> FKAERLRVNLRLVINRLKLLEKKKTELAQKARKEIADYLAAGKDERARIRVEHIIREDYLVEAMEILELYCDLLLARFGLIQSMKELDSGLAESVSTLIWAAPRLQSEVAELKIVADQLCAKYSKEYGKLCRTNQIGTVNDRL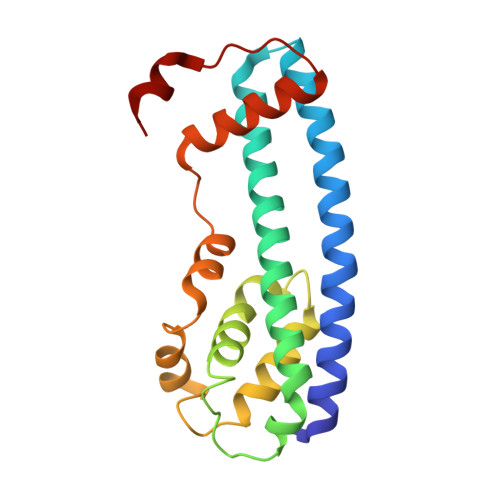MHKLSVEAPPKILVERYLIEIAKNYNVPYEPDSVVMAEA NORBIOTIN | 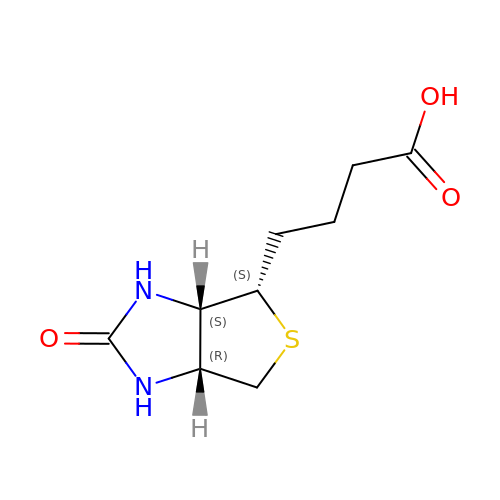C9 H14 N2 O3 S | AINAXQHKYSZESH-HAFWLYHUSA-N>MKKFTCVQDIGDLKSALAESFEIKKDRFKYVELGRNKTLLMIFFNSSLRTRLSTQKAALNLGMNVIVLDINQGAWKLETERGVIMDGDKPEHLLEAIPVMGCYCDIIGVRSFARFENREYDYNEVIINQFIQHSGRPVFSMEAATRHPLQSFADLITIEEYKKTARPKVVMTWAPHPRPLPQAVPNSFAEWMNATDYEFVITHPEGYELDPKFVGNARVEYDQMKAFEGADFIYAKNWAAYTGDNYGQILSTDRNWTVGDRQMAVTNNAYFMHCLPVRRNMIV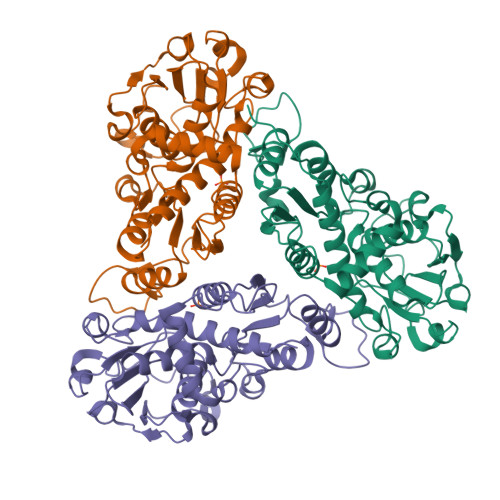TDDVIESPQSIVIPEAANREISATVVLKRLLENLPHHHHHH[3x]> MNVTIYDVAREASVSMATVSRVVNGNPNVKPSTRKKVLETIERLGYRPNAVARGLASKKTTTVGVIIPDISNIFYAELA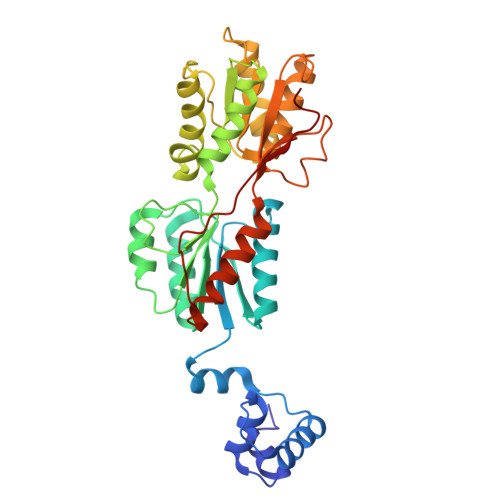RGIEDIASMYKYNIILSNSDQNQDKQLHLLNNMLGKQVDGIIFMSGNVTEEHVEELKKSPVPVVLAASIESTNQIPSVTIDYEQAAFDAVQSLIDSGHKNIAFVSGTLEEPINHAKKVKGYKRALTESGLPVRDSYIVEGDYTYDSGIEAVEKLLEEDEKPTAIFVGTDEMALGVIHGAQDRGLNVPNDLEIIGFDNTRLSTMVRPQLTSVVQPMYDIGAVAMRLLTKYMNKETVDSSIVELPHRIEFRQSTK>MRGDGDGWVMSENGARFWGRHGAAGLLLRAPMPGGAAAVLLQHRAPWSHQGGTWALPG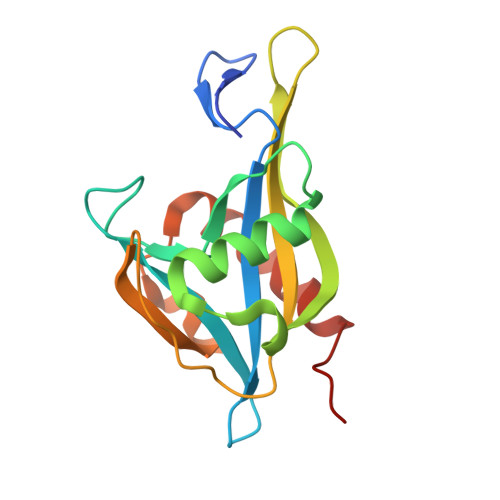GARDSHETPEQAAVRAAHAAAGLPAEQLTVRTTVVTAEVAGIGGTQWTYTTVIADAAEPLHTVPNRESAELRWVLEDQVADLPLHPGFAASWQRLREVTATIPLLNRQR[2x]> DEYSYYKLKGASTQLEYTKYMASTLQEIAQRFPDLQNTGILQDLENYNKAWNDFASNPNENATKIALVKASQTLTESVNNTFATLDKIQKKVNDDIKNTVDEINRIGEEIATINKQIYGQEALPTEHANELRDRRDELELTLSKLVSAVASKNEINQDNRLDTTITDPGHQYNLSIEGFSIVDGINFHPLKLDYDDKNKSYSIYYETPDEKVRDLTAKISGGQLGAQLDLRGRNYSKSEGKYEDGIIQGYMDSLDTFAKTMINETNNLYASSAKSSVTSDYLSGLKGDIPLVNYDRTIQPGSFDIVIYDDKGDKKLTKTITIDVNTTMNDIMRQINANTDDNDNKNSNDDVDDHINASFSYDAKTGDGLFQINAKSGFKVAIEDKGTNFAGAFSIGGFFSGTDASDMKVKDSILNDPSTVRASSNGVDSGNDMANKIIQLQYKKVNFYNEDGTIDNLTMEEYYRKLTGKIASDGENNNVVNSSNETLYNSVYSEYQSKSGVNTNEELAALI

A special junction to assure a smooth connectivity is needed to link the hook and the filament, which have different structural and functional characteristics. In this junction, the first segment, composed of the FlgK complex, is in contact with the hook, while the second segment, made by the FlgL complex, connects to the filament. The junctions made by FlgK and FlgL play important roles in bridging the hook to the filament. Once the hook is completed, FlgK starts appearing at the top of the hook to form the first junction, followed by FlgL that builds up at the top of the ring made of FlgK.

Here, we solved the three-dimensional structure of a major fragment of FlgK from C. jejuni, strain ATCC 700819/NCTC 11168, using X-ray crystallography. To crystallize FlgK (67 kDa) of C. jejuni strain ATCC 700819/NCTC 11168, we removed 68 and 28 amino acid residues from the N- and C- termini, respectively. The remaining 58 kD fragment, named FlgKcj58, has 511 amino acids (See Methods for detailed experimental procedures). The crystal belongs to the orthorhombic space group P21212 and it diffracted to 2.45 Å resolution. The structure of FlgKcj58, in which 11 C-terminal residues were not resolved, comprises the fragment [Asp69-Gly568]. FlgKcj58 can be described as composed of two domains. There is a central domain, D1, which could be divided into two sub domains, D1a and D1b, and a more compact domain D2, consisting mostly of β-strands. The structure of FlgKcj58 reveals that the cell-proximal half of the protein, which includes the N- and C- termini, and which is known to connect to the hook, is structurally conserved when compared with other known FlgK protein structures. However, the cell-distal half of the protein has diverged, developing a different 3D structure. Domain D2 of FlgKcj58 has a different fold compared to domains D2 of FlgKse49 and of FlgKbp64.> MGGGGGGALNKLFPGYKDKIWMKVPVQWRQQMIQHWNKSYEKQVYSESVALNRTFQARNQLVLDRLKPSGAYRLPAVDYKR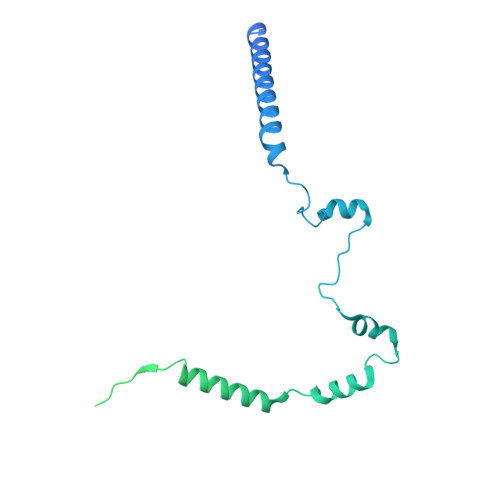QLSRGTLVEGADFYLPTAQEQQRLARHFEPYSEQEQEERRKFRFQSISVYLAVALGASFVHDYFYQRRPVAWCLEKEPPHPPSYPFWFKSLFHSHDIPSVRRGYEVYRKVCATCHSMEQLHFRHLVGEVLPEKRVKQIAAEYDVTDGPNDQGEMYTRPGILGDAFPSPYPNEEAARYANGGAYPPDLSLITAARHFGPDYLMALLGGYRDPPEGVELRPGLYWNVWFPGNAIAMPPPLMDEMIDYEDGTPCNISQMSKDVVNFLTWATEPTADERKLYGLKCVSAIAIGTVLMTLWWRFYWAMYATRRIDFGKLKYL>MTTELNQGEQFVADFRANAAALTTANAYNPEDEHDACGVGFIAAIDGKPRRSVVEKGIEALKAVWHRGAVDADGKTGDGAGIHVAVPQKFFKDHVKVIGHRAPDNKLAVGQVFLPRISLDAQEACRCIVETEILAFGYYIYGWRQVPINVDIIGEKANATRPEIEQIIVGNNKGVSDEQFELDLYIIRRRIEKAVKGEQINDFYICSLSARSIIYKGMFLAEQLTTFYPDLLDERFESDFAIYHQRYSTNTFPTWPLAQPFRMLAHNGEINTVKGNVNWMKAHETRMEHPAFGTHMQDLKPVIGVGLSDSGSLDTVFEVMVRAGRTAPMVKMMLVPQALTSSQTTPDNHKALIQYCNSVMEPWDGPAALAMTDGRWVVGGMDRNGLRPMRYTITTDGLIIGGSETGMVKIDETQVIEKGRLGPGEMIAVDLQSGKLYRDRELKDHLATLKPWDKWVQNTTHLDELVKTASLKGEPSDMDKAELRRRQQAFGLTMEDMELILHPMVEDGKEAIGSMGDDSPIAVLSDKYRGLHHFFRQNFSQVTNPPIDSLRERRVMSLKTRLGNLGNILDEDETQTRLLQLESPVLTTAEFRAMRDYMGDTAAEIDATFPVDGGPEALRDALRRIRQETEDAVRGGATHVILTDEAMGPARAAIPAILATGAVHTHLIRSNLRTFTSLNVRTAEGLDTHYFAVLIGVGATTVNAYLAQEAIAERHRRGLFGSMPLEKGMANYKKAIDDGLLKIMSKMGISVISSYRGGGNFEAIGLSRALVAEHFPAMVSRISGIGLNGIQKKVLEQHATAYNEEVVALPVGGFYRFRKSGDRHGWEGGVIHTLQQAVTNDSYTTFKKYSEQVNKRPPMQLRDLLELRSTKAPVPVDEVESITAIRKRFITPGMSMGALSPEAHGTLNVAMNRIGAKSDSGEGGEDPARFRPDKNGDNWNSAIKQVASGRFGVTAEYLNQCRELEIKVAQGAKPGEGGQLPGFKVTEMIARLRHSTPGVMLISPPPHHDIYSIEDLAQLIYDLKQINPDAKVTVKLVSRSGIGTIAAGVAKANADIILISGNSGGTGASPQTSIKFAGLPWEMGLSEVHQVLTLNRLRHRVRLRTDGGLKTGRDIVIAAMLGAEEFGIGTASLIAMGCIMVRQCHSNTCPVGV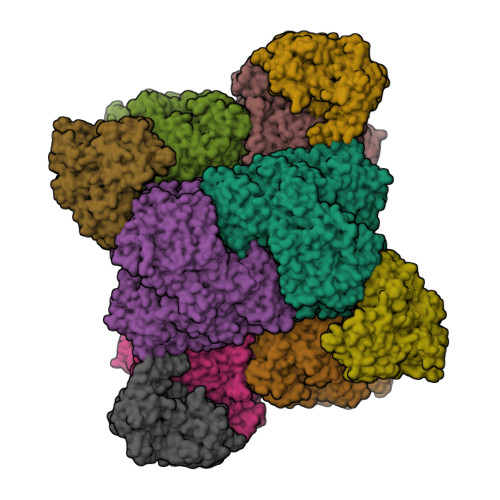CVQDDKLRQKFVGTPEKVVNLFTFLAEEVREILAGLGFRSLNEVIGRTDLLHQVSRGAEHLDDLDLNPRLAQVDPGENARYCTLQGRNEVPDTLDARIVADARPLFEEGEKMQLAYNARNTQRAIGTRLSSMVTRKFGMFGLQPGHITIRLRGTAGQSLGAFAVQGIKLEVMGDANDYVGKGLSGGTIVVRPTTSSPLETNKNTIIGNTVLYGATAGKLFAAGQAGERFAVRNSGATVVVEGCGSNGCEYMTGGTAVILGRVGDNFAAGMTGGMAYVYDLDDSLPLYINDESVIFQRIEVGHYESQLKHLIEEHVTETQSRFAAEILNDWAREVTKFWQVVPKEMLNRLEVPVHLPKAISAE[6x];>MANQRMLGFVHTAQRMPDKRPAAERRQDFAEIYARFSDERANEQANRCSQCGVPFCQVHCPVSNNIPDWLKLTSEGRLEEAYEVSQATNNFPEICGRICPQDRLCEGNCVIEQSTHGAVTIGSVEKYINDTAWDQGWVKPRTPSRELGLSVGVIGAGPAGLAAAEELRAKGYEVHVYDRYDRMGGLLVYGIPGFKLEKSVVERRVKLLADAGVIYHPNFEVGRDASLPELRRKHVAVLVATGVYKARDIKAPGSGLGNIVAALDYLTTSNKVSLGDTVEAYENGSLNAAGKHVVVLGGGDTAMDCVRTAIRQGATSVKCLYRRDRKNMPGSQREVAHAEEEGVEFIWQAAPEGFTGDTVVTGVRAVRIHLGVADATGRQTPQVIEGSEFTVQADLVIKALGFEPEDLPNAFDEPELKVTRWGTLLVDHRTKMTNMDGVFAAGDIVRGASLVVWAIRDGRDAAEGIHAYAKAKAEAPVAVAAE[4x]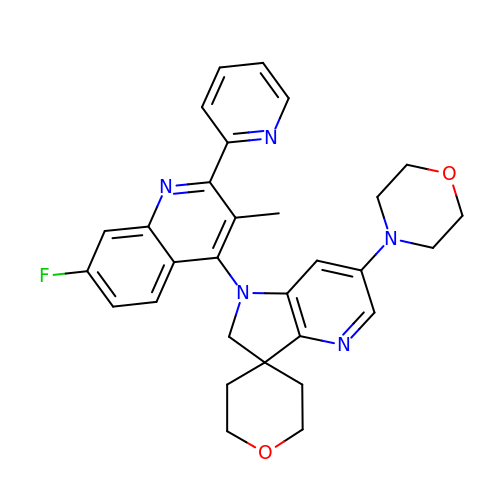1'-[7-fluoro-3-methyl-2-(pyridin-2-yl)quinolin-4-yl]-6'-(morpholin-4-yl)-1',2,2',3,5,6-hexahydrospiro[pyran-4,3'-pyrrolo[3,2-b]pyridine] | C30 H30 F N5 O2 | JZYCUVQYCHLFBL-UHFFFAOYSA-N>MEAVPRMPMIWLDLKEAGDFHFQPAVKKFVLKNYGENPEAYNEELKKLELLRQNAVRVPRDFEGCSVLRKYLGQLHYLQSRVPMGSGQEAAVPVTWTEIFSGKSVAHEDIKYEQACILYNLGALHSMLGAMDKRVSEEGMKVSCTHFQCAAGAFAYLREHFPQAYSVDMSRQILTLNVNLMLGQAQECLLEKSMLDNRKSFLVARISAQVVDYYKEACRALENPDTASLLGRIQKDWKKLVQMKIYYFAAVAHLHMGKQAEEQQKFGERVAY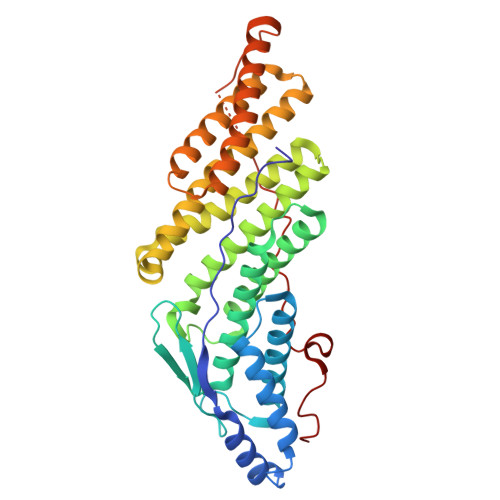FQSALDKLNEAIKLAKGQPDTVQDALRFTMDVIGGKYNSAKKDNDFIYHEAVPALDTLQPVKGAPLVKPLPVNPTDPAVTGPDIFAKLV[2x];> KKKEEEDDDMKELENWAGSM> SLK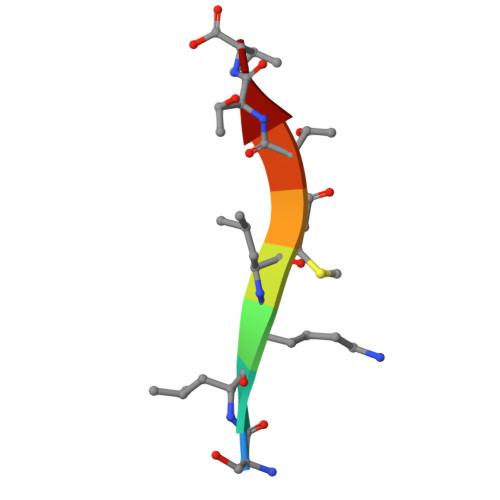LMTTV>MSINQLTLAVASDQEISAHGYPTMSDAVEHFSSSASHGFKDCRFVAFGLQDIVIGVEPSDFVVALEGDEILTAYIATFGARPRCLRGWLIPSNSNYVLEEFQVIFGKRGGLEHHHHHHHH[2x]

Similar to β-CoV nsp1, α-CoV nsp1 has been identified as an important virulence factor that acts by inhibiting the host protein synthesis function. Here, we are the first to report a 1.8-Å full-length crystal structure for FIPV nsp1 and a 2.1-Å full-length crystal structure of SADS-CoV nsp1. The crystal structures of SADS-CoV nsp1 and FIPV nsp1 reveal that their monomers contain six antiparallel β-strands and two α-helices. The overall structure of α-CoVs nsp1 shared the same fold, with a characteristic six-stranded β-barrel formed by β1 relative to β6, β2 relative to β5, and β3 relative to β4.

As a newly discovered CoV, SADS-CoV broke out in 2017 in Guangdong Province, causing the death of approximately 25,000 piglets within a few months. The SADS-CoV nsp1 and FIPV nsp1 structures were refined to 2.1- and 1.8-Å resolutions, respectively. Their space groups are P212121 and C121, respectively. Each asymmetric unit of SADS-CoV nsp1 and the FIPV nap1 structures contained two and four subunits, respectively. With the exception of the regions encompassing amino acids 105 to 110 of SADS-CoV nsp1 and 106 to 110 of FIPV nsp1, all the residues of both nsp1 proteins can be built using the final models. Similarly, structure comparison showed that the overall structure of SADS-CoV nsp1 is conserved relative to that of PEDV nsp1 (with an RMSD of 0.84 Å), but it has several differences relative to TGEV nsp1 (with an RMSD of 1.89 Å). For SADS-CoV nsp1 and PEDV nsp1, the length of the β6 is significantly shorter in SADS-CoV nsp1. Additionally, there are also substantial differences in the loops, especially those located at residues 11 to 22 in SADS-CoV nsp1. Furthermore, the structures of α-CoV 1A nsp1s and α-CoV 1B nsp1s also exhibit obvious differences in some loops, especially those located at residues 52 to 59 in SADS-CoV nsp1. Specifically, SADS-CoV nsp1 and PEDV nsp1 have a wider distribution of negative charges on the surface than FIPV nsp1 and TGEV nsp1.>[4x]MAHHHHHHSSGLEVLFQGPMWVDFSDTASMKNLDPQGGFKVGTVFKKEISPGYVVTLTVTELKPFNSTEIYKKRVEGTPTANTYD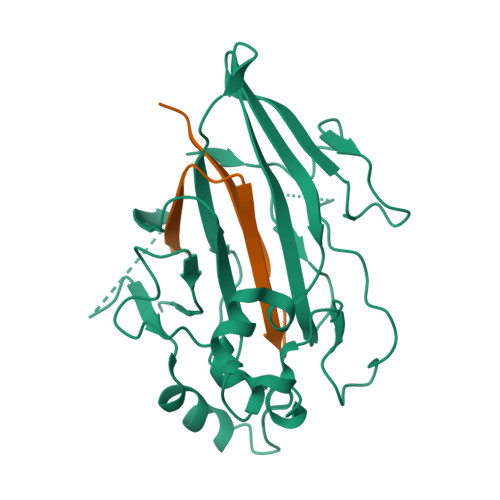PNAINSYLKGYKDYGKTPPSVTGRPQNKFSTIGGQGFDTQGRKTQIILPDDAVNWGIKFKVEATYRGNPVKPSVVMADGEDANPAEYGIFTTNGEGWEYVGEWMKGPRAKGPYTVMTEDMVKAFDKTRKDGLLILKDKSVDWSKYLSPDTVTGGLGSQVFGPIISASKAVPVVMTRGASEVGFYVATGGQQALMMGFLVVDSSDAPASYGEAYHTIGTRDSIANTPINQPYLGSTAADIDADSESDWTADDRE> AGIQKDSTGKCGPPPPIDNGDITSFPLSVYAPASSVEYQCQNLYQLEGNKRITCRNGQWSEPPKCLHPCVISREIMENYNIALRWTA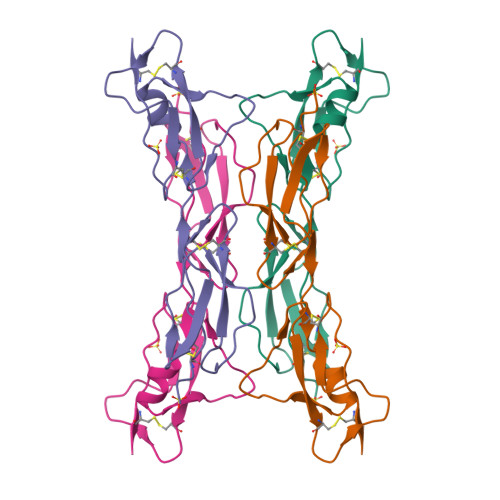KQKLYSRTGESVEFVCKAGYRLSSRSHTLRTTCWDGKLEYPTCAKR>DDVPPRIARAMENEEYWDFDIFELEAATHNRPLIYLGLKMFARFGICEFLHCSESTLRSWLQIIEANYHSSNPYHNSTHSADVLHATAYFLSKERIKETLDPIDEVAALIAATIHDVDHPGRTNSFLCNAGSELAILYNDTAVLESHHAALAFQLTTGDDKCNIFKNMERNDYRTLRQGIIDMVLATEMTKHFEHVNKFVNSINKPLATLEENGETDKNQEVINTMLRTPENRTLIKRMLIKCADVSNPCRPLQYCIEWAARISEEYFSQTDEEKQQGLPVVMPVFDRNTCSIPKSQISFIDYFIT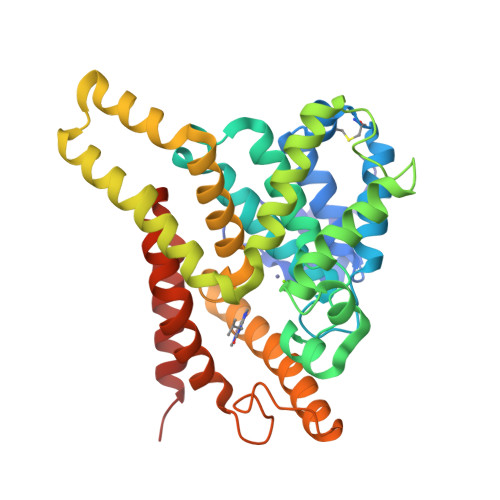DMFDAWDAFVDLPDLMQHLDNNFKYWKGLDEM[2x]>ATYAMMLIENVEYDVLLERFKKILRQGGLKYTKQREVLLKTLYHSDTHYTPESLYMEIKQA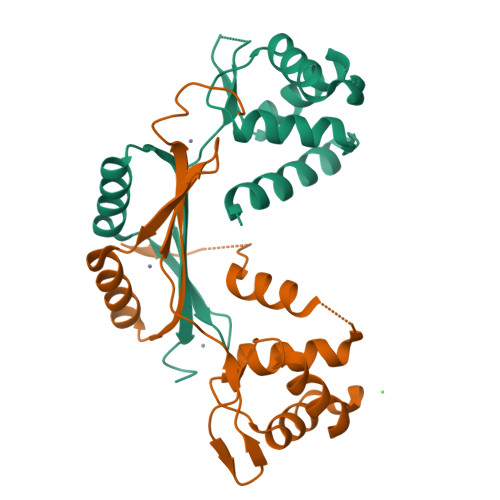EPDLNVGIATVYRTLNLLEEAEMVTSISFGSAGKKYELANKPHHDHMICKNCGKIIEFENPIIERQQALIAKEHGFKLTGHLMQLYGVCGDCNNQKAKVKI[2x]In N. gonorrhoeae, the best characterized and most clinically important multidrug efflux system that mediates multidrug resistance (MDR) is the multiple transferrable resistance (Mtr)CDE tripartite efflux pump. MtrD works in conjunction with the MtrC periplasmic membrane fusion protein and MtrE outer membrane channel to actively export antimicrobials out of bacterial cells. The cryo-EM structure of MtrDCR103 revealed that this multidrug efflux pump adopts the overall fold of hydrophobe-amphiphile efflux (HAE)-RND-type proteins and forms a homotrimer. Each protomer contains 12 transmembrane helices (TM1 to TM12) and a large periplasmic domain, which can be divided into six subdomains (PN1, PN2, PC1, PC2, DN, and DC).

To elucidate how MtrDCR103 recognizes macrolide antibiotics in solution, we incubated a 2-μM MtrDCR103-nanodisc sample with 10 μM Ery for 2 hours to form the MtrDCR103-Ery complex. We determined a cryo-EM structure of this complex to a resolution of 2.72 Å. The overall structure of MtrDCR103-Ery is almost identical to that of Amp bound (labeled as MtrDCR103-Amp), with the three protomers displaying the access, binding, and extrusion forms. In the binding protomer of MtrDCR103, the cryo-EM images depict that an additional large density corresponding to the bound Ery drug was found at the distal multidrug binding site. It is somewhat surprisingly that the observed large Ery molecule is anchored within this deep pocket. The binding of Ery is extensive; within 4.5 Å of this bound drug, there are seven aromatic, two hydrophobic, two polar, and one positively charged residues that provide aromatic stacking and hydrophobic and electrostatic interactions to facilitate Ery binding. These important binding residues are F136, I139, R174, F176, S275, T277, Y325, F568, V607, F610, F612, and F623. The MtrDCR103 periplasmic binding cleft is able to accommodate Ery and forms additional electrostatic and hydrophobic contacts with R174, Y325, F568, and F623. Likewise, the cryo-EM structure of the MtrDCR103-Ery complex depicts that there are 23 PE lipids that are similarly oriented as the lipids in the Amp-bound structure.

>[3x]MAKFFIDRPIFAWVISIFIIAAGIFGIKSLPVSQYPSVAAPTITLHAIYPGASAQVMEGSVLSVIERNMNGVEGLDYMSTSADSSGSGSVSLTFTPDTDENLAQVEVQNKLSEVLSTLPATVQQYGVTVSKARSNFLMIVMLSSDVQSTEEMNDYAQRNVVPELQRIEGVGQVRLFGAQRAMRIWVDPKKLQNYNLSFADVGSALSAQNIQISAGSIGSLPAVRGQTVTATVTAQGQLGTAEEFGNVILRANTDGSNIYLKDVAKVGLGMEDYSSSTRLNGVNTTGMAVMLSNSGNAMATAKAVKERLAVLEKYFPQGMSWKTPYDTSKFVEISIEKVIHTLIEAMVLVFVVMYLFLQNIRYTLIPTIVVPISLLGGFAFISYMGMSINVLTMFAMILVIGIVVDDAIVVVENVERIMAGEGLPPKEATKKAMGQISGAVIGITAVLISVFVPLAMFSGAAGNIYKQFALTMASSIAFSAFLALTLTPALCATMLKTIPKGHHEEKKGFFGWFNKKFDSWTHGYEGRVAKVLRKTFRMMVVYIGLAVVGVFLFMRLPTSFLPTEDQGFVMVSVQLPAGATKERTDATLAQVTQLAKSIPEIENIITVSGFSFSGSGQNMAMGFAILKDWNERTASGSDAVAVAGKLTGMMMGTLKDGFGIAVVPPPILELGNGSGLSINLQDRNNTGHTALLAKRNELIQKMRASGLFDPSTVRAGGLEDSPQLKIDINRAAAAAQGVSFADIRTALASALSSSYVSDFPNQGRLQRVMVQADGDARMQPADILNLTVPNSSGIAVPLSSIATVSWQMGTEQSVRFNGYPAMELSGSPATGVSTGQAMEAVQKMVDELGSGYSLEWGGQSREEAKGGSQTIALYALAAVAVFLVLAALYESWSIPLAVLLVMPLGLAGAAAGVTGRNLFEGLLGSVPSFANDIYFQVGFVTVMGLSAKNAILIIEFAKDLQAQGKSAVEAALEAARLRFRPIIMTSFAFILGVVPLYIAGGASSASQRAIGTTVFWGMLIGTLLSVFLVPLFYVVVRKFFKETAHE To bypass this protective barrier, some phages encode polysaccharide-degrading enzymes referred to as depolymerases to provide access to cell surface receptors. Here, we characterized the structure and enzymatic activity of DpK2, showing it to be a capsule-degrading hydrolase specific for K2-type polysaccharides. Based largely on homology modeling, but supported by recent structural analyses, depolymerase RBPs are modular, comprising three functional domains: an N-terminal domain that tethers it to the phage baseplate or to other elements of the tail, a central β-helical domain that contains the enzymatic activity of the protein, and a C-terminal domain which may either act as an autochaperone or, in some cases, form a noncatalytic carbohydrate binding module. While the archetypal siphoviruses such as Lambda, T1, T5, and Chi use “L-shaped” or fibrous appendages on their tails to bind cell surface features, phage RAD2 has globular appendages comprised of the depolymerase RBP DpK2.

To investigate the mechanism by which the RBP capsule depolymerase functions, DpK2 was purified as an enzymatically active trimer and its structure solved at a resolution of 2.7 Å. Initial reconstructions using C1 symmetry revealed an elongated molecule of approximately 180 Å (18 nm) in length, consistent with the dimensions of the tail appendages measured in the initial TEM micrographs of the RAD2 virion. Three discernible domains of DpK2 could be observed: an N-terminal domain containing an extended triple helical bundle, a central beta-helical domain, and a distinct C-terminal domain. C3 symmetry was used to further refine the structure of DpK2 to 2.7 Å resolution. Residues 191 to 906 of DpK2 could be modeled within the electron density. However, due to the applied C3 symmetry, high-resolution structural information of the N-terminal triple helical bundle was lost. The central domain (residues 317 to 642) is formed by three parallel right-handed β-helices consisting of 10 rungs, with each helix of the trimer being formed by an individual monomer. Analysis of the surface properties of DpK2 revealed a prominent negatively charged cavity (yellow oval) located within the central β-helical domain at the interface between neighboring monomers. Adjacent grooves (yellow lines) were observed emanating from the cavity, which may facilitate binding to or funneling of substrates toward the active site. This cavity consists of a negatively charged triad (D543, E545, and D546) and two dyads (D399-E423 and D619-E620) within close proximity, suggesting that DpK2 may function as a hydrolase. However, structural differences were observed in the C-terminal domain of DpK2, which consists of a β-sandwich fold followed by a far C-terminal α-helical bundle.

>[3x]MALYREGKAAMAADGTVTGTGTKWQSSLSLIRPGATIMFLSSPIQMAVVNKVVSDTEIKAITTSGAVVASTDYAILLSDSLTVDGLAQDVAETLRHYQSQETVIADAVEFFKSFDFDSLQNLANQIKADSESAESSAAAAAASESKAKTSEDNAKSSENAAKNSEVAAETTRDQIQQIIDNAGDQSTLVVLAQPDGFDSIGRVSSFAALRNLKPKKSGQHVLLTSYYDGWAAENKMPTGGGEFISSIGTATDDGGYIAAGPGYYWTRVVNNNSFTAEDFGCKTTATPPPNFNVLPAELFDNTAMMQAAFNLAISKSFKLNLSTGTYYFESSDTLRITGPIHIEGRPGTVFYHNPSNKANPKTDAFMNISGCSAGRISSINCFSNSYLGKGINFDRSVGDNRKLVLEHVYVDTFRWGFYVGEPECINQIEFHSCRAQSNYFQGIFIESFKEGQEYGHSAPVHFFNTICNGNGPTSFALGATYKTTKNEYIKVMDSVNDVGCQAYFQGLSNVQYIGGQLSGHGSPRNTSLATITQCNSFIIYGTDLEDINGFTTDGTAITADNIDAIESNYLKDISGAAIVVSSCPGFKIDSPHIFKIKTLSTIKLMNNTYNYEIGGFTPDEALKYNVWDANGLATNRISGVIHPRLVNSRLGINSVAFDNMSNKLDVSSLIHNETSQIVGLTPSTGSNVPHTRKMWSNGAMYSSTDLNNGFRLNYLSNHNEPLTPMHLYNEFSVSEFGGSVTESNALDEIKYIFIQTTYANSGDGRFIIQALDASGSVLSSNWYSPQSFNSTFPISGFVRFDVPTGAKKIRYGFVNSANYTGSLRSHFMSGFAYNKRFFLKIYAVYNDLGRYGQFEPPYSVAIDRFRVGDNTTQMPSIPASSATDVAGVNEVINSLLASLKANGFMSS The 2-oxoglutarate (2OG) dependent hypoxia inducible factor (HIF) prolyl hydroxylases (PHDs) are targets for treatment of anaemia and other ischaemia related diseases. Prolyl hydroxylation of HIF-α subunits signals for their degradation via the ubiquitin–proteasome system. Inhibition of the human HIF-α prolyl hydroxylases (PHD1-3) has the potential to mimic elements of the physiological hypoxic response. We report structure–activity relationship and crystallographic studies on spiro[4.5]decanone containing PHD inhibitors.

To inform the SAR work, crystal structures of tPHD2 in complex with our 1,3,8-triazaspiro[4.5]decane-2,4-dione compound series were pursued. We obtained a structure of tPHD2 in complex with 11 and MnII (substituting for FeII) (S2 and S4 and Table S3†). The new structure reveals that 11 makes similar interactions with PHD2 to those observed for 17.13 The 3-methyl pyridine ring of 11 penetrates into the 2OG binding pocket. The active site metal is chelated by the tertiary amine of the piperidine ring and 3-methyl pyridinyl nitrogen of 11. The biphenyl substituent of 11 is positioned in an aromatic pocket formed by the Trp-258, Trp-389 and Phe-391 side-chains, with which it makes hydrophobic/π-stacking interactions. The terminal phenyl ring of the biphenyl substituent of 11 is positioned to form a cation π-interaction with the catalytically important residue Arg-322.17,18 Arg-322 is also positioned to hydrogen bond to the imidazolidine-2,4-dione ring of 11. The pyrimidine ring of 11, which is not present in 17, is positioned to form a π-stacking interaction with the phenol ring of Tyr-310. The 3-hydroxypyridine derivatives 38, 41 and 44 were produced because analysis of the PHD2 structure in complex with 11 suggested that replacing the methyl group of 11 with a hydroxyl group may form additional interactions with PHD2, via hydrogen bonding to either Tyr-310 or Tyr-303. The inhibition results with these derivatives reveal the pyrimidine ring has a minor role in enabling potent tPHD2 inhibition, i.e. the non-pyrimidine containing analogues 23 are only somewhat weaker compared to 11 (IC5011, 0.253 μM; 23, 0.741 μM). Prior analyses of truncated PHD2 in complex with a spiro[4.5]decanone inhibitor reveal a binding mode involving chelation of the active site metal (Mn(ii) was substituted for Fe(ii) to produce a complex stable for crystallization) via the tertiary amine of its piperidine ring and a pyridinyl nitrogen.13 Chelation of the active site metal of 2OG oxygenases by a pyridine ring is well precedented, e.g. with pyridine carboxylate inhibitors.

> GSHMASPNGQTKPLPALKLALEYIVPCMNKHGICVVDDFLGKETGQQIGDEVRALHDTGKFTDGQLVSQKSDSSKDIRGDKITWIEGKEPGCETIGLLMSSMDDLIRHCNGKLGSYKINGRTKAMVACYPGNGTGYVRHVDNPNGDGRCVTCIYYLNKDWDAKVSGGILRIFPEGKAQFADIEPKFDRLLFFWSDRRNPHEVQPAYATRYAITVWYFDADERARAKVKYLTGE>MGSSHHHHHHSQDPMLKTNIELKPKVEAFLNEEIKMFINGEFVSAIGGKTFETYNPATEDVLAVVCEAQEEDIDAAVKAARSAFESGPWAEMTTAERAHLIYKLADLIEEHREELAQLEALDNGKPYQVALDDDISATVENYRYYAGWTTKIIGQTIPISKDYLNYTRHEPVGVVGQIIPWNFPLVMSSWKMGAALATGCTIVLKPAEQTPLSLLYAAKLFKEAGFPNGVVNFVPGFGPEAGA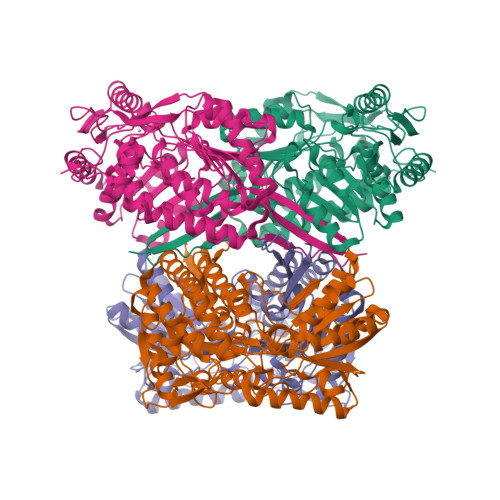AIVNHHDIDKVAFTGSTVTGKYIMRQSAEMIKHVTLELGGKSPNIILEDADLEEAINGAFQGIMYNHGQNCSAGSRVFVHRKHYETVVDALVKMANNVKLGAGMEKETEMGPLVSKKQQERVLNYIEQGKKEGATVAAGGERALEKGYFVKPTVFTDVTDDMTIVKEEIFGPVVVVLPFDSTEEVIERANNSSYGLAAGVWTQNIKTGHQVANKLKAGTVWINDYNLENAAAPFGGYKQSGIGRELGSYALDNYTEVKSVWVNIK[4x]L-N(OMEGA)-NITROARGININE-(4R)-AMINO-L-PROLINE AMIDE | C11 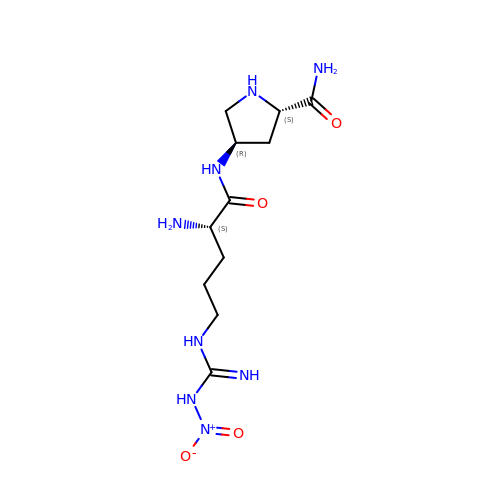H22 N8 O4 | IUFRDGFKAVLPFZ-CSMHCCOUSA-N Kelch repeat and BTB domain-containing protein 4 (KBTBD4) is the substrate receptor of a cullin3-dependent E3 ligase complex (CRL3KBTBD4). Recurrent indel mutations in the Kelch domain of the KBTBD4 E3 ligase rewire epigenetic programs for stemness in medulloblastoma by recruiting LSD1-CoREST-HDAC1/2 complexes as neo-substrates for ubiquitination and degradation. UM171, an investigational drug for haematopoietic stem cell transplantation, was found to degrade LSD1-CoREST-HDAC1/2 complexes in a wild-type KBTBD4-dependent manner, suggesting a potential common mode of action. The mutant and drug-induced complexes adopt similar structural assemblies requiring both Kelch domains in the KBTBD4 dimer for each HDAC2 interaction.

To determine the structure of the lower affinity KBTBD4WT complex mediated by UM171, we used the BS3 crosslinker to stabilise the binding of the CoREST1NT2-HDAC2 neo-substrate. This sample yielded 2:2 and 2:1 KBTBD4WT-UM171-HDAC2 complexes at 2.9 Å and 3.1 Å, respectively. No such density was found in the 2:2 complex, likely due to steric constraints that would prevent CoREST1 binding in this higher order assembly. The cryo-EM datasets for the KBTBD4WT-UM171-HDAC2 complexes yielded 2:1 and 2:2 models displaying an RSMD value of 1.55 Å across 1055 Cα positions. Superposition of the 2:1 and 2:2 states shows that the high structural conservation extends across the protein-compound and protein-protein interaction sites, indicating that the neo-substrate recruitment mechanism in these complexes is conserved regardless of the stoichiometry. UM171 is buried in the site 1 interfaces where it forms contacts with blades II and III from the KBTBD4WT Kelch domain, as well as with the HDAC2 catalytic pocket. The methyl tetrazole inserts into the HDAC2 catalytic pocket to form extensive interactions, including a hydrogen bond with HDAC2 Y304 and π–π interactions with HDAC2 F151, F206 and H179. The binding is further stabilised by π–π interactions between the buried UM171 pyrimidoindole core and HDAC2 residues F151 and F206. Outside of the HDAC2 catalytic pocket, UM171 forms hydrophobic interactions with KBTBD4WT I310 and P311 from the BC II loop and L356 located at the tip of the BC III loop. Site 1 superposition reveals that UM171 mimics the mutated BC II loop of KBTBD4R313PRR by engaging the same HDAC2 residues in its catalytic pocket.

>[2x]MESPEEPGASMDENYFVNYTFKDRSHSGRVAQGIMKLCLEEELFADVTISVEGREFQLHRLVLSAQSCFFRSMFTSNLKEAHNRVIVLQDVSESVFQLLVDYIYHGTVKLRAEELQEIYEVSDMYQLTSLFEECSRFLARTVQVGNCLQVMWLADRHSDPELYTAAKHCAKTHLAQLQNTEEFLHLPHRLLTDIISDGVPCSQNPTEAIEAWINFNKEEREAFAESLRTSLKEIGENVHIYLIGKESSRTHSLAVSLHCAEDDSISVSGQNSLCHQITAACKHGGDLYVVGGSIPRRMWKCNNATVDWEWCAPLPRDRLQHTLVSVPGKDAIYSLGGKTLQDTLSNAVIYYRVGDNVWTETTQLEVAVSGAAGANLNGIIYLLGGEENDLDFFTKPSRLIQCFDTETDKCHVKPYVLPFAGRMHAAVHKDLVFIVAEGDSLVCYNPLLDSFTRLCLPEAWSSAPSLWKIASCNGSIYVFRDRYKKGDANTYKLDPATSAVTVTRGIKVLLTNLQFVLA;>MAYSQGGGKKKVCYYYDGDIGNYYYGQGHPMKPHRIRMTHNLLLNYGLYRKMEIYRPHKATAEEMTKYHSDEYIKFLRSIRPDNMSEYSKQMQRFNVGEDCPVFDGLFEFCQLSTGGSVAGAVKLNRQQTDMAVNWAGGLHHAKKSEASGFCYVNDIVLAILELLKYHQRVLYIDIDIHHGDGVEEAFYTTDRVMTVSFHKYGEYFPGTGDLRDIGAGKGKYYAVNFPMRDGIDDESYGQIFKPIISKVMEMYQPSAVVLQCGADSLSGDRLGCFNLTVKGHAKCVEVVKTFNLPLLMLGGGGYTIRNVARCWTYETAVALDCEIPNELPYNDYFEYFGPDFKLHISPSNMTNQNTPEYMEKIKQRLFENLRMLPHAPGVQMQAIPEDAVHEDSGDEDGEDPDKRISIRASDKRIACDEEFSDSEDEGEGGRRNVADHKKGAKKARIEEDKKETEDKKTDVKEEDKSKDNSGEKTDTKGTKSEQLSNP[2x]> SDSQQSIKVLEELFQKLSVATADNRHEIASEVASFLNGNIIEHDVPEHFFGELAKGIKDKKTAANAMQAVAHIANQSNLSPSVEPYIVQLVPAICTNAGNKDKEIQSVASETLISIVNAVNPVAIKALLPHLTNAIVETNKWQEKIAILAAFSAMVDAAKDQVALRMPELIPVLSETMWDTKKEVKAAATAAMTKATETVDNKDIERFIPSLIQCIADPTEVPETVHLLGATTFVAEVTPATLSIMVPLLSRGLNERETGIKRKSAVIIDNMCKLVEDPQVIAPFLGKLLPGLKSNFATIADPEAREVTLRALKTLRRVGNVGEDDAIPELSHAGDVSTTLQVVNELLKDETVAPRFKIVVEYIAAIGADLIDERIIDQQAWFTHITPYMTIFLHEKKAKDILDEFRKRAVDNIPVGPNFDDEEDEGEDLCNCEFSLAYGAKILLNKTQLRLKRARRYGICGPNGCGKSTLMRAIANGQVDGFPTQEECRTVYVEHDIDGTHSDTSVLDFVFESGVGTKEAIKDKLIEFGFTDEMIAMPISALSGGWKMKLALARAVLRNADILLLDEPTNHLDTVNVAWLVNYLNTCGITSITISHDSVFLDNVCEYIINYEGL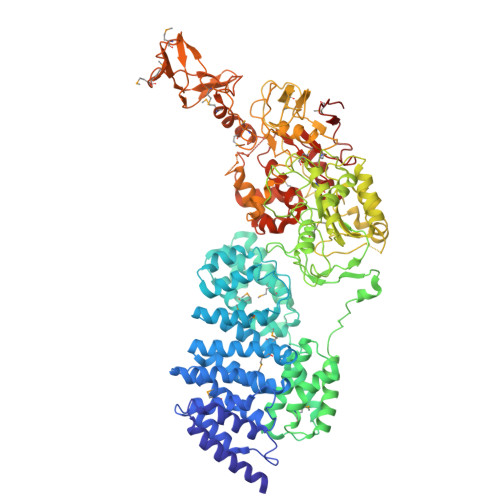KLRKYKGNFTEFVKKCPAAKAYEELSNTDLEFKFPEPGYLEGVKTKQKAIVKVTNMEFQYPGTSKPQITDINFQCSLSSRIAVIGPNGAGKSTLINVLTGELLPTSGEVYTHENCRIAYIKQHAFAHIESHLDKTPSEYIQWRFQTGEDRETMDRANRQINENDAEAMNKIFKIEGTPRRIAGIHSRRKFKNTYEYECSFLLGENIGMKSERWVPMMSVDNAWIPRGELVESHSKMVAEVDMKEALASGQFRPLTRKEIEEHCSMLGLDPEIVSHSRIRGLSGGQKVKLVLAAGTWQRPHLIVLDEPTNYLDRDSLGALSKALKEFEGGVIIITHSAEFTKNLTEEVWAVKDGRMTPSGHN>[2x]MSAFDYDLFVIG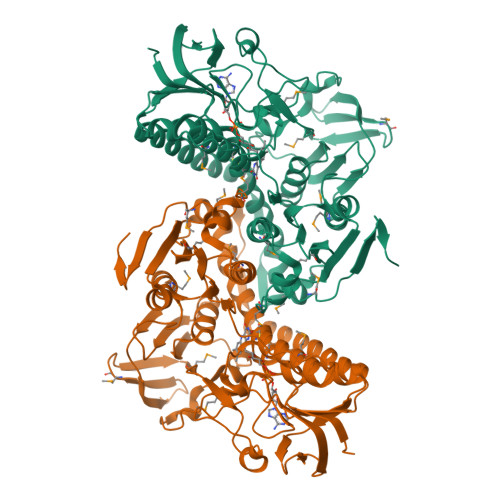GGSGGVRSGRLAAALGKKVAIAEEFRYGGTCVIRGCVPKKLYVYASQFAEHFEDAAGFGWTVGESRFDWAKLVAAKEQEIARLEGLYRKGLANAGAEILDTRAELAGPNTVKLLASGKTVTAERIVIAVGGHPSPHDALPGHELCITSNEAFDLPALPESILIAGGGYIAVEFANIFHGLGVKTTLIYRGKEILSRFDQDMRRGLHAAMEEKGIRILCEDIIQSVSADADGRRVATTMKHGEIVADQVMLALGRMPNTNGLGLEAAGVRTNELGAIIVDAFSRTSTPGIYALGDVTDRVQLTPVAIHEAMCFIETEYKNNPTSPDHDLIATAVFSQPEIGTVGITEEEAARKFQEIEVYRAEFRPMKATLSGRKEKTIMKLVVNAADRKVVGAHILGHDAGEMAQLLGISLRAGCTKDDFDRTMAVHPTAAEELVTMYQPSYRVRNGERVG> MSLISKEELIKLAYSIRPRENEYKTILTNLDEYNKLTTNNNENKYLQLKKLNESIDVFMNKYKTSSRNRALSNLKKDILKEVILIKNSNTSPVEKNLHFVWIGGEVSDIALEYIKQWADINAE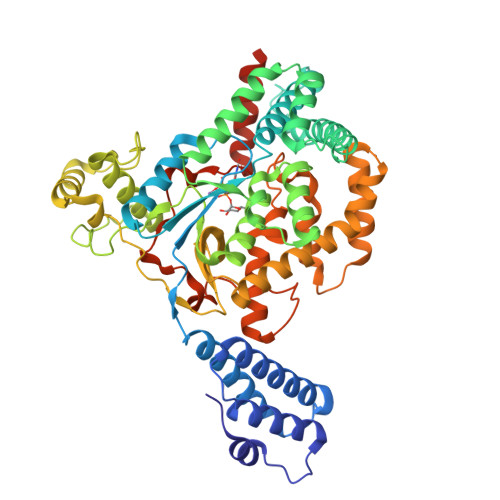YNIKLWYDSEAFLVNTLKKAIVESSTTEALQLLEEEIQNPQFDNMKFYKKRMEFIYDRQKRFINYYKSQINKPTVPTIDDIIKSHLVSEYNRDETVLESYRTNSLRKINSNHGIDIRANSLFTEQELLNIYSQELLNRGNLAAASDIVRLLALKNFGGVYLDVDMLPGIHSDLFKTISRPSSIGLDRWEMIKLEAIMKYKKYINNYTSENFDKLDQQLKDNFKLIIESKSEKSEIFSKLENLNVSDLEIKIAFALGSVINQALISKQGSYLTNLVIEQVKNRYQFLNQHLNPAIESDNNFTDTTKIFHDSLFNSATAENSMFLTKIAPYLQVGFMPEARSTISLSGPGAYASAYYDFINLQENTIEKTLKASDLIEFKFPENNLSQLTEQEINSLWSFDQASAKYQFEKYVRDYTGGSLHAGLRGSHHHHHH> MVAPKPKPAHEQVEPALIPSNWTSVIPLLTSDFKNQYSVISRLKNPNMKPVPYAGDIIKLMAFINKFSSFFHSDLQNLSFQDFEVGLDLYPGDPNGSAAGIVKGPEDTSLLLYPDFMAIKDIVYCQDKMNLLFLSLLDLTFTE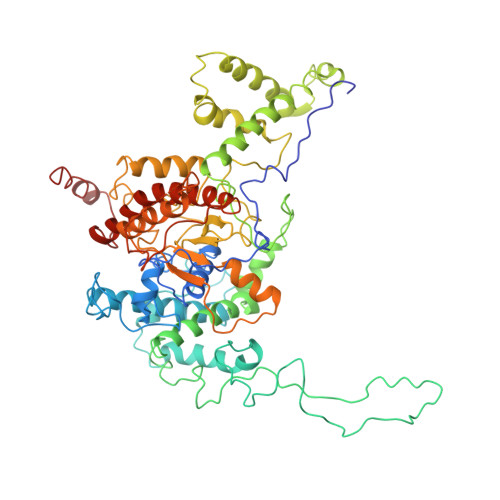NFDGKSAKKKGPLTTWENLKSSSKKVFSNPLYRLRLVAREWGYPREWRQQLPSDQDISKPKTALFEQDEQTPVVDPSHPEILTPNIYTWNANEPLPLESNPLYNREMDKNGILALKPMDRVVLLRALTDWCASHSSAIHDEIYKLTHGKKDPVFGIQTQQVPRYTIEGVDNTINQFKKLCSLIQSRYEIRSKKKHFVKQLKEGKKPDLSRKLEILKEIKAELKNAVKSEKDELLFSLYDKWVPLFEGELPDQPLANPFSERLYKLRLQEFFLGRVPHIGDFYMPRLHSYGDSLEMSTFTDLRNLQALLSKFKNNEYNAFTLFENDGQSMSAQFKLFYHDTPSLAHDVARGRNTSGKVYWYELCHDSATLLEFLEFLDYKIVKPQDEKKEGNEKEKEALNNEAHILEQKSTTDNNPSINTNPLPKDAKYNTARKKLQILKEFLSDYYFILRQFEQMKVQFADMKPGKRQLRRIQRQTVNYNT> MTVKKLYFIPAGRCMLDH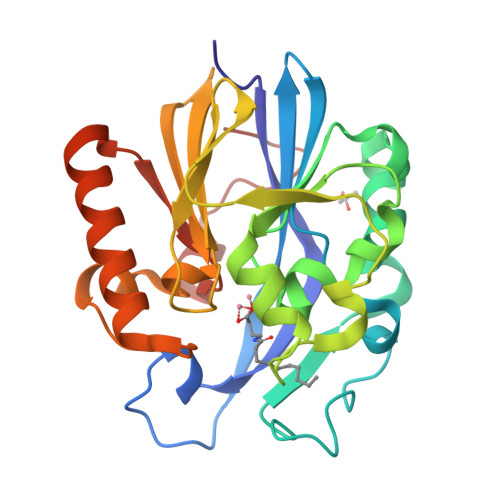SSVNSALTPGKLLNLPVWCYLLETEEGPILVDTGMPESAVNNEGLFNGTFVEGQILPKMTEEDRIVNILKRVGYEPDDLLYIISSHLHFDHAGGNGAFTNTPIIVQRTEYEAALHREEYMKECILPHLNYKIIEGDYEVVPGVQLLYTPGHSPGHQSLFIETEQSGSVLLTIDASYTKENFEDEVPFAGFDPELALSSIKRLKEVVKKEKPIIFFGHDIEQEKSCRVFPEYI> VIVPEGTQLDEKQHIVINNGAEPQSFDPHKTEGVPESNVAYQLLEGLVTSDSEGKLQPGAAESWENTPDFKTWTFHLRKDAKWSNGDPVTAHDFVFAWRRLVDPATAAPYASYLSYLQVENAQDIIDGKKKPAELGVEAKDDYTFVVHATNPVPYAVSLTTHQSLLPLPQKVVEKLGDAWVKKENYVGNGAYKLANHIINEKIEFERNPLYWNDKETVINSATFLAIENPSTDVARYRAGDLDMTSYGLPPEQFAKLKKELLGEVYVTRTLGTYSYELNNKKAPFDNVNIRKALNL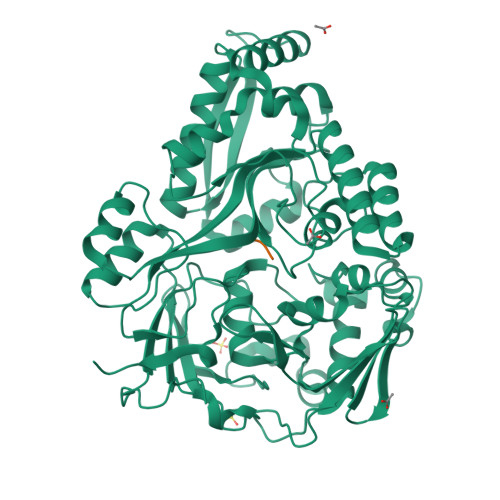SLDRNVITDKVLGQGQTPTYVFTPTYIEEGHLIQQPAYSKEPMAQRNEEAIKLLEEAGYSKANPLKFSILYNTNENHKKVAIAAASMWKANTKGLIDVKLENQEWKTYIDSRRAGRYDVARAGWHADYNQATTFGNYFLSNSSNNTAKYANPEYDKAMAESYAATDAEGRAKAYAKAEEILGKDYGIVPIFNYVNPRLVKPYVKGYSGKDPQDHIYLRNLYIIKH;> AAAA> GPGSMAAGRAQVPSSEQAWLEDAQVFIQKTLCPAVKEPNVQLTPLVIDCVKTVWLSQGRNQGSTLPLSYSFVSVQDLKTHQRLPCCSHLSWSSSAYQAWAQEAGPNGNPLPREQLLLLGTLTDLSADLEQECRNGSLYVRDNTGVLSCELIDLDLSWLGHLFLFPRWSYLPPARWNSSGEGHLELWDAPVPVFPLTISPGPVTPIPVLYPESASCLLRLRNKLRGVQRNLAGSLVRLSALVKSKQKAYFILSLGRSHPAVTHVSIIVQVPAQLVWHRALRPGTAYVLTELRVSKIRGQRQHVWMTSQSSRLLLLKPECVQELELELEGPLLEADPKPLPMPSNSEDKKDPESLVRYSRLLSYSGAVTGVLNEPAGLYELDGQLGLCLAYQQFRGLRRVMRPGVCLQLQDVHLLQSVGGGTRRPVLAPCLRGAVLLQSFSRQKPGAHSSRQAYGASLYEQLVWERQLGLPLYLWATKALEELACKLCPHVLRHHQFLQHSSPGSPSLGLQLLAPTLDLLAPPGSPVRNAHNEILEEPHHCPLQKYTRLQTPSSFPTLATLKEEGQRKAWASFDPKALLPLPEASYLPSCQLNRRLAWSWLCLLPSAFCPAQVLLGVLVASSHKGCLQLRDQSGSLPCLLLAKHSQPLSDPRLIGCLVRAERFQLIVERDVRSSFPSWKELSMPGFIQKQQARVYVQFFLADALILPVPRPCLHSATPSTPQTDPTGPEGPHLGQSRLFLLCHKEALMKRNFCVPPGASPEVPKPALSFYVLGSWLGGTQRKEGTGWGLPEPQGNDDNDQKVHLIFFGSSVRWFEFLHPGQVYRLIAPGPATPMLFEKDGSSCISRRPLELAGCASCLTVQDNWTLELESSQDIQDVLDANKSLPESSLTDLLSDNFTDSLVSFSAEILSRTLCEPLVASLWMKLGNTGAMRRCVKLTVALETAECEFPPHLDVYIEDPHLPPSLGLLPGARVHFSQLEKRVSRSHNVYCCFRSSTYVQVLSFPPETTISIPLPHIYLAELLQGGQSPFQATASCHIVSVFSLQLFWVCAYCTSICRQGKCTRLGSTCPTQTAISQAIIRLLVEDGTAEA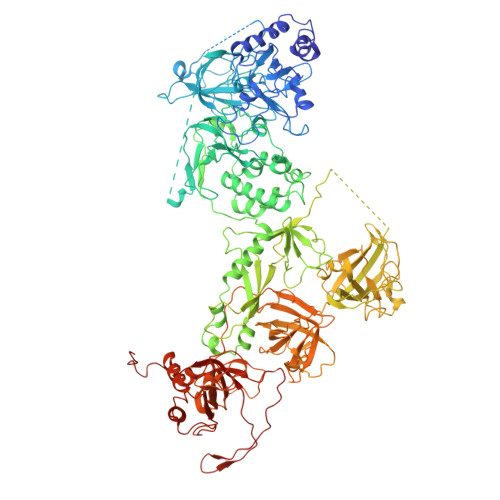VVTCRNHHVAAALGLCPREWASLLDFVQVPGRVVLQFAGPGAQLESSARVDEPMTMFLWTLCTSPSVLRPIVLSFELERKPSKIVPLEPPRLQRFQCGELPFLTHVNPRLRLSCLSIRESEYSSSLGILASSC>MFERFTDRARRVVVLAQEEARMLNHNYIGTEHILLGLIHEGEGVAAKSLESLGISLEGVRSQVEEIIGQGQQAPSGHIPFTPRAKKVLELSLREALQLGHNYIGTEHILLGLIREGEGVAAQVLVKLGAELTRVRQQVIQLLSGYQGKEAAEAGTGGRGGESGSPSTSLVLDQFGRNLTAAAMEGKLDPVIGREKEIERVMQVLSRRTKNNPVLIGEPGVGKTAVVEGLAQAIVHGEVPETLKDKQLYTLDLGSLVAGSRYRGDFEERLKKVLKEINTRGDIILFIDELHTLVGAGAAEGAIDAASILKPKLARGELQTIGATTLDEYRKYIEKDAALERRFQPVQVGEPTVEHTIEILKGLRDRYEAHHRVSITDAAMVAAATLADRYINDRFLPDKAIDLIDEAGARMRIRRMTAPPDLREFDEKIAEARREKESAIDAQDFEKAASLRDREKTLVAQRAEREKQWRSGDLDVVAEVDDEQIAEVLGNWTGIPVFKLTEAETTRLLRMEEELHKRIIGQEDAVKAVSKAIRRTRAGLKDPKRPSGSFIFAGPSGVGKTELSKALANFLFGDDDALIQIDMGEFHDRFTASRLFGAPPGYVGYEEGGQLTEKVRRKPFSVVLFDEIEKAHQEIYNSLLQVLEDGRLTDGQGRTVDFKNTVLIFTSNLGTSDISKPVGLGFSKGGGENDYERMKQKVNDELKKHFRPEFLNRIDDIIVFHQLTREEIIRMVDLMISRVAGQLKSKDMALVLTDAAKALLAKRGFDPVLGARPLRRTIQREIEDQLSEKILFEEVGPGQVVTVDVDNWDGEGPGEDAVFTFTGTRKPPAEPDLAKAGAHSAGGPEPAARLEHHHHHH[6x]

The unfoldase ClpC1 is one of the most exciting drug targets against tuberculosis. This AAA+ unfoldase works in cooperation with the ClpP1P2 protease and is the target of at least four natural product antibiotics: cyclomarin, ecumicin, lassomycin, and rufomycin. ClpC1 is a member of the class II AAA+ family of proteins, which contains an N-terminal domain (NTD) and two distinct ATP-binding modules, D1 and D2. While ClpP alone is able to rapidly hydrolyze peptides, the degradation of large proteins requires the presence of a hexameric AAA+ ATPase complex, such as ClpX or ClpC1. These ATPases activate the Clp proteases but also bind protein substrates, unfold them, and translocate them into the proteolytic compartment.

To further stabilize the sample, considering that ATP is being continuously degraded even at low temperatures and that some AAA+ proteins have been shown to hydrolyze ATP analogs, we introduced two additional mutations in the double walker B motif (E288A and E626A). We hypothesized that these mutations allow nucleotide binding but prevent hydrolysis and therefore further stabilize the hexameric assembly. After initial cryo-EM grid screening, a dataset was collected of the apo form of MtbClpC1E288A/F444A/E626A (see Experimental procedures). Processing of the data resulted in a structure for apo ClpC1 determined to a resolution of 3.6 Å (see Experimental procedures). As expected, the overall structure of apo MtbClpC1E288A/F444A/E626A consists of a hexamer composed of six ClpC1 subunits (A–F), with the D1 and D2 domains arranged in a ring that together forms a pore through which the substrate can be actively translocated. In line with recent structures, including the recent cryo-EM structure of B. subtilis ClpC, the observed ClpC1 hexamer is not symmetric, as observed originally in the crystal structure of ClpC, and instead adopts an asymmetric spiral structure. An important characteristic of our structure is the observation of a 23-residue long peptide visible in its central pore. The presence of substrates in the pore formed by D1 and D2 has been previously reported for other members of the family, but as no substrate has been added to our cryo-EM sample preparation, it was probably taken up and trapped inside of the inactive protein during purification. Furthermore, all nucleotide-binding sites in D1 are occupied by ADP, while for D2, four sites are occupied by ADP (subunits B, C, D, and E), while two are in their apo state (subunits A and F). Finally, the NTD and its adjacent 26 residue linker are not visible in our apo ClpC1 structure.> NDDLWHQWKRMYNKEYNGADDQHRRNIWEKNVKHIQEHNLRHDLGLVTYTLGLNQFTDMTFEEFKAKYLTEMSRASDILSHGVPYEANNRAVPDKIDWRESGYVTEVKDQGNCGSGWAFSTTGTMEGQYMKNERTSISFSEQQLVDCSRPWGNNGCGGGLMENAYQYLKQFGLETESSYPYTAVEGQCRYNKQLGVAKVTGFYTVHSGSEVELKNLVGAEGPAAVAVDVESDFMMYRSGIYQSQTCSPL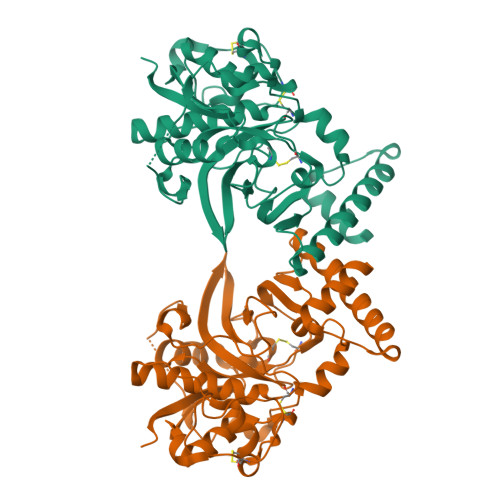RVNHAVLAVGYGTQGGTDYWIVKNSWGLSWGERGYIRMVRNRGNMCGIASLASLPMVARFP> KDTELR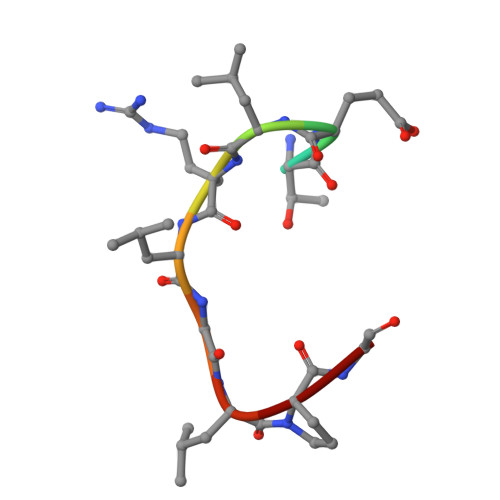LGLPG>HMERLLDELTLEGVARYMQSERCRRVICLVGAGISTSAGIPDFRSPSTGLYDNLEKYHLPYPEAIFEISYFKKHPEPFFALAKELYPGQFKPTICHYFMRLLKDKGLLLRCYTQNIDTLERIAGLEQEDLVEAHGTFYTSHCVSASCRHEYPLSWMKEKIFSEVTPKCEDCQSLVKPDIVFFGESLPARFFSCMQSDFLKVDLLLVMGTSLQVQPFASLISKAPLSTPRLL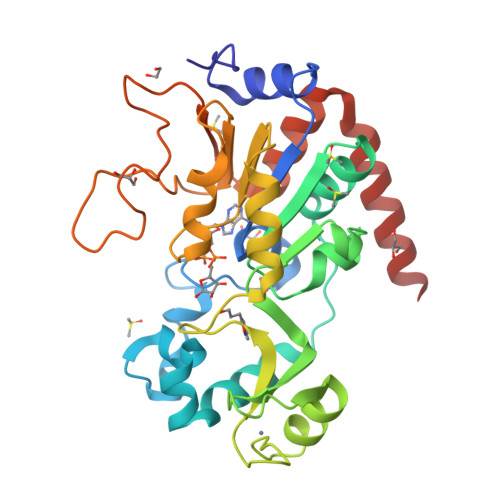INKEKAGQSDPFLGMIMGLGGGMDFDSKKAYRDVAWLGECDQGCLALAELLGWKKELEDLVRREHASIDAQS[2x]>[4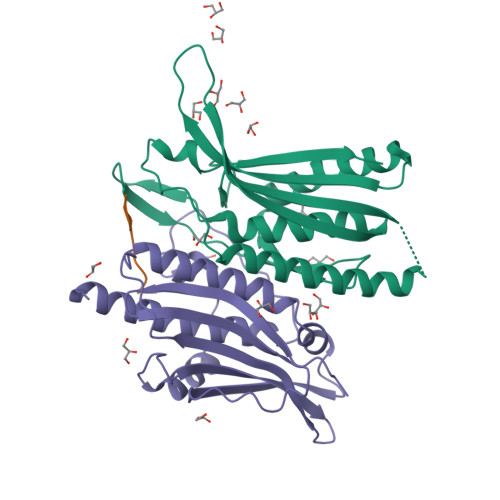x]GGTSEDELPPQVHKVGSDEAMNCRSEVLEVSVEGRQVEEAMLAVLHTVLLHRSTGKFHYKKEGTYSIGTVGTQDVDCDFIDFTYVRVSSEELDRALRKVVGEFKDALRNSGGDGLGQMSLEFYQKKKSRWPFSDECIPWEVWTVKVHVVALATEQERQICREKVGEKLCEKIINIVEVMNRHEYLPKMPTQSEVDNVFDTGLRDVQPYLYKISFQITD;>[2x]METDLNSQDRKDLDKFIKFFALKTVQVIVQARLGEKICTRSSSSPTGSDWFNLAIKDIPEVTHEAKKALAGQLPAVGRSMCVEISLKTSEGDSMELEIWCLEMNEKCDKEIKVSYTVYNRLSLLLKSLLAITRVTPAYRLSRKQGHEYVILYRIYFGEVQLSGLGEGFQTVRVGTVGTPVGTITLSCAYRINLAFMS> GSHMKNSVSVDLPGSMKVLVSKSSNADGKYDLIATVDALELSGTSDKNNGSGVLEGVKADASKVKLTISDDLGQTTLEVFKSDGSTLVSKKVTSNGSSTEEKFNEKGEVSEKIITRADGTRLEYTGIKSDGSGKAKEVLKGYVLEGTLTAEKTTLVVKEGTVTLSKNISKSGEVSVELNDTDSSAATKKTAAWNS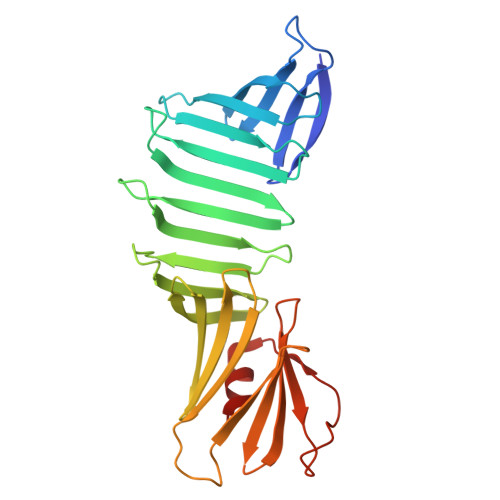GTSTLTITVNSKKTKDLVFTSSNTITVQQYDSNGTSLEGSAVEITKLDEIKNALK> MSFINYSSREINCKIVYYGPGLCGKTTNLQYIYNKTAAETKGKLISLSTETDRT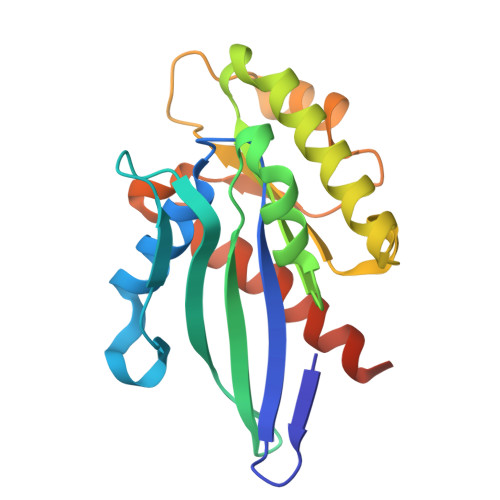LFFDFLPLSLGEIRGFKTRFHLYTVPGQVFYDASRKLILKGVDGVVFVADSQIERMEANMESLENLRINLAEQGYDLNKIPYVIQYNKRDLPNAVTVEEMRKALNHRNIPEYQAVAPTGVGVFDTLKAVAKLVLTELKKGGGSHHHHHH>MGDTKEQRILRYVQQNAKPGDPQSVLEAIDTYCTQKEWAMNVGDAKGQIMDAVIREYSPSLVLELGAYCGYSAVRMARLLQPGARLLTMEINPDCAAITQQMLNFAGLQDKVTILNGASQDLIPQLKKKYDVDTLDMVFLDHWKD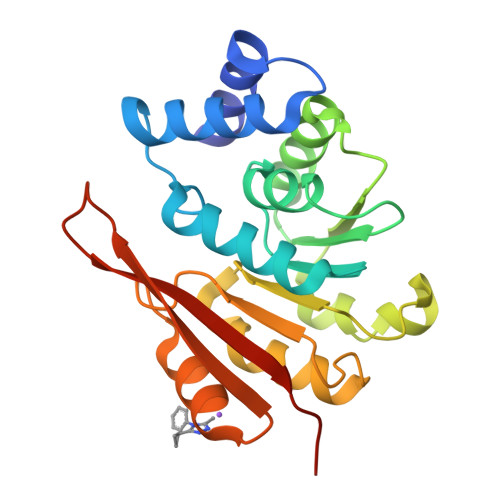RYLPDTLLLEKCGLLRKGTVLLADNVIVPGTPDFLAYVRGSSSFECTHYSSYLEYMKVVDGLEKAIYQGPSSPDKS[4x]> ARLNITFSPQAFEDYKYFQQNNKKMVKKINELLKSIDRNGALEGIGKPEKLKSNLTGYYSRRINHEHRLVYTV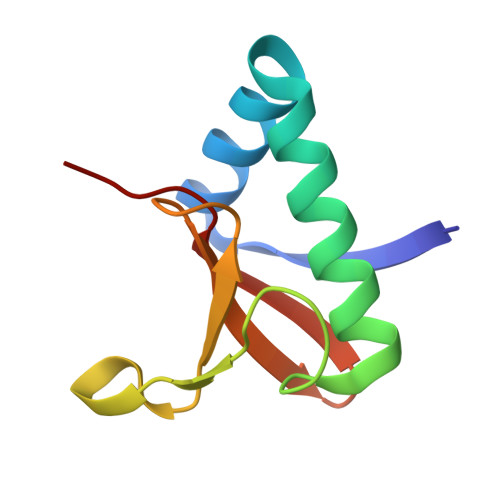DDNHIKIASCKYHY>MQDNSRYTHFLTQHY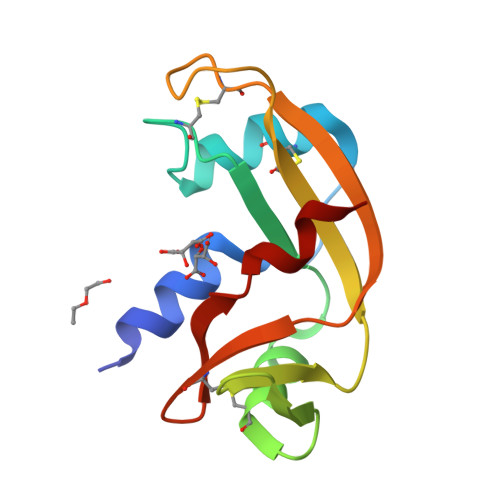DAKPQGRDDRYCESIMRRRGLTSPCKDINTFIHGNKRSIKAICENKNGNPHRENLRISKSSFQVTTCKLHGGSPWPPCQYRATAGIRNVVVACENGLPVHLDQSIFRRP[2x]> MAEDADMRNELEEMQRRADQLADESLESTRRMLQLVEESKDAGIRTLVMLDEQGEQLER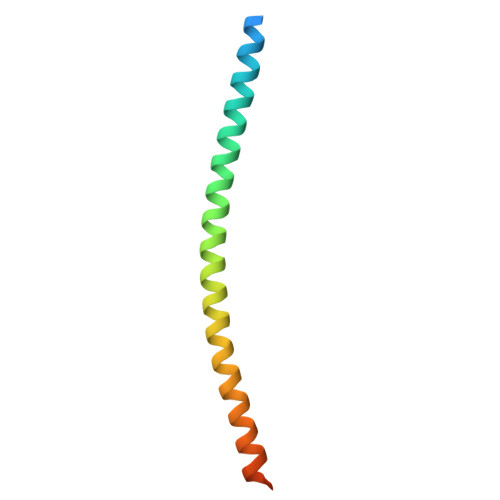IEEGMDQINKDMKEAEKNLTDLG> MVRIVIDSGVDSGRPIGVVPFQWAGPGAAPEDIGGIVAADLRNSGKFNPLDRARLPQQPGSAQEVQPAAWSALGIDAVVVGQVTPNPDGSYNVAYQLVDTGGAPGTVLAQNSYKVNKQWLRYAGHTASDEVFEKLTGIKGAFRTRIAYVVQTNGGQFPYELRVSDYDGYNQFVVHRSPQCLMSPAWSPDGSKLAYVTFESGR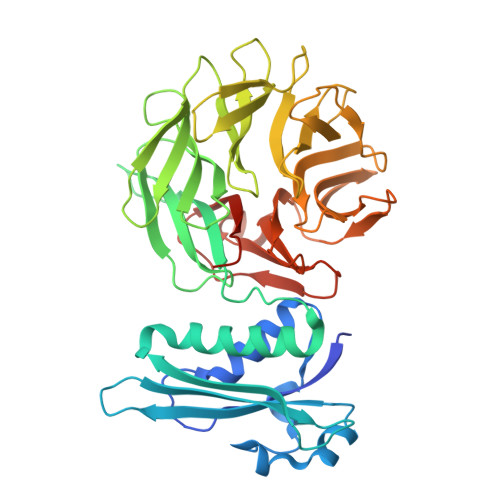SALVIQTLANGAVRQVASFPRHNGAPAFSPDGSKLAFALSKTGSLNLYVMDLASGQIRQVTDGRSNNTEPTWFPDSQNLAFTSDQAGRPQVYKVNINGGAPQRITWEGSQNQDADVSSDGKFMVMVSSNGGQQHIAKQDLATGGVQVLSSTFLDETPSLAPNGTMVIYSSSQGMGSVLNLVSTDGRFKARLPATDGQVKFPAWSPYLLEHHHHHH7-[[[3-[(dimethylamino)methyl]phenyl]amino]methyl]quinolin-2-amine | C19 H22 N4 | 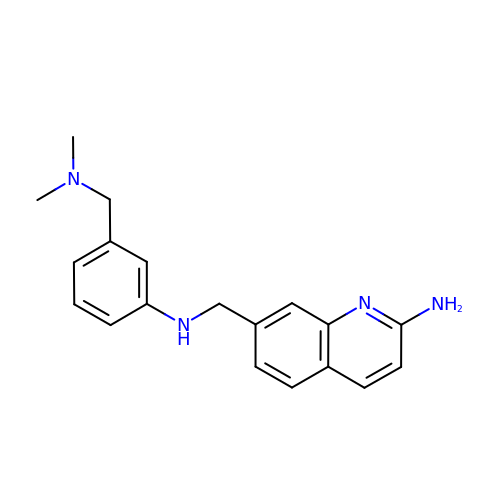KLVQNBMBSWDRJZ-UHFFFAOYSA-N Uridine-Diphosphate-Methylene-N-acetyl-galactosamine | C18 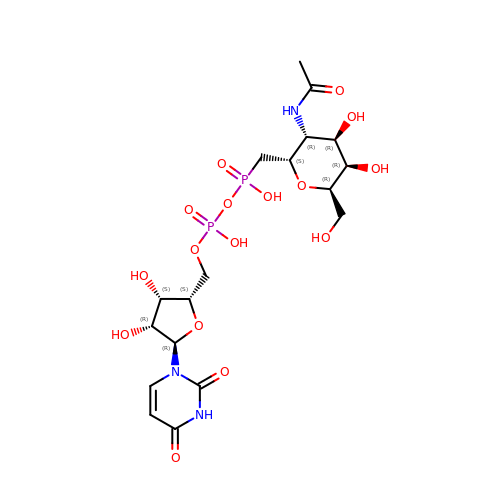H29 N3 O16 P2 | KUFKOJZYUNOEES-HCUIDVLSSA-N> MGGVAMPGAEDDVVRENLYFQGKDGLAAMENAHTKTVEEVLGHFGVNESTGLSLEQVKKLKERWGSNELPAEEGKTLLELVIEQFEDLLVRILLLAACISFVLAWFEEGEETITAFVEPFVILLILVANAIVGVWQERNAENAIEALKEYEPEMGKVYRQDRKSVQRIKAKDIVPGDIVEIAVGDKVPADIRLTSIKSTTLRVDQSILTGESVSVIKHTDPVPDPRAVNQDKKNMLFSGTNIAAGKAMGVVVATGVNTEIGKIRDEMVATEQERTPLQQKLDEFGEQLSKVISLICIAVWIINIGHFNDPVHGGSWIRGAIYYFKIAV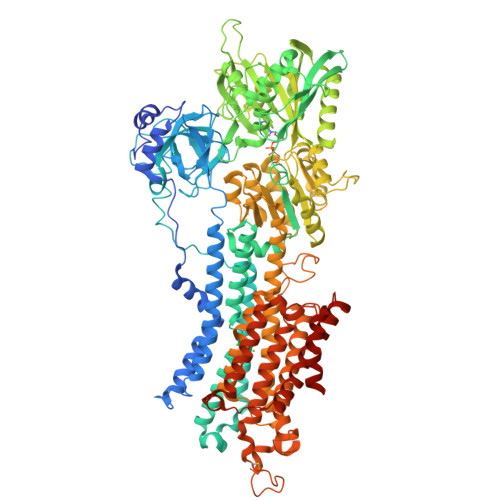ALAVAAIPEGLPAVITTCLALGTRRMAKKNAIVRSLPSVETLGCTSVICSDKTGTLTTNQMSVCRMFILDRVEGDTCSLNEFTITGSTYAPIGEVHKDDKPVNCHQYDGLVELATICALCNDSALDYNEAKGVYEKVGEATETALTCLVEKMNVFDTELKGLSKIERANACNSVIKQLMKKEFTLEFSRDRKSMSVYCTPNKPSRTSMSKMFVKGAPEGVIDRCTHIRVGSTKVPMTSGVKQKIMSVIREWGSGSDTLRCLALATHDNPLRREEMHLEDSANFIKYETNLTFVGCVGMLDPPRIEVASSVKLCRQAGIRVIMITGDNKGTAVAICRRIGIFGQDEDVTSKAFTGREFDELNPSAQRDACLNARCFARVEPSHKSKIVEFLQSFDEITAMTGDGVNDAPALKKAEIGIAMGSGTAVAKTASEMVLADDNFSTIVAAVEEGRAIYNNMKQFIRYLISSNVGEVVCIFLTAALGFPEALIPVQLLWVNLVTDGLPATALGFNPPDLDIMNKPPRNPKEPLISGWLFFRYLAIGCYVGAATVGAAAWWFIAADGGPRVSFYQLSHFLQCKEDNPDFEGVDCAIFESPYPMTMALSVLVTIEMCNALNSLSENQSLLRMPPWENIWLVGSICLSMSLHFLILYVEPLPLIFQITPLNVTQWLMVLKISLPVILMDETLKFVARNYLEPGKECVQPATKSCSFSACTDGISWPFVLLIMPLVIWVYS5-[(2-phenylethyl)sulfanyl]-2-{[(4-phenylpiperazin-1-yl)sulfonyl]amino}benzoic 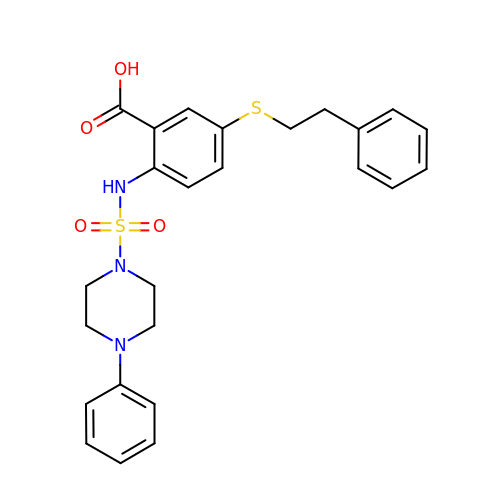acid | C25 H27 N3 O4 S2 | DTSFWGSGVLNQNG-UHFFFAOYSA-N> MSGQFTGTGTGGDVFKVDLNEQFDRADMVWIGTASVLVWIMIPGVGLLYSGISRKKHALSLMWAALMAACVAAFQWFWWGYSLVFAHNGSVFLGTLQNFCLKDVLGAPSIVKTVPDILFCLYQGMFAAVTAILMAGAGCERARLGPMMVFLFIWLTVVYCPIAYWTWGGNGWLVSLGALDFAGGGPVHENSGFAALAYSLWLGKRHDPVAKGKVPKYKPHSVSSIVMGTIFLWFGWYGFNGGSTGNSSMRSWYACVNTNLAAATGGLTWMLVDWFRTGGKWSTVGLCMGAIAGLVGITPAAGYVPVYTSVIFGIVPAIICNFAVDLKDLLQIDDGMDVWALHGVGGFVGNFMTGLFAADYVAMIDGTEIDGGWMNHHWKQLGYQLAGSCAVAAWSFTVTSIILLAMDRIPFLRIRLHEDEEMLGTDLAQIGEYAYYADDDPETNPYVLEPIRSTTISQPLPHIDGVADGSSNNDSGEAKNHHHHHH

structures of the Mep2 transceptors from S. cerevisiae and C. albicans. function as ammonium receptors/sensors in fungal development. a central channel for the transport of ammonium. non-phosphorylated, with channels that are closed on the cytoplasmic side.

different crystal forms to high resolution (up to 1.5 Å). Mep2 channel closure is likely due to movements of the CTR and ICL1 and ICL3. twin-His motif via hydrogen bonding with a highly conserved tyrosine hydroxyl group. the region beyond Ser457 is disordered. should facilitate the phosphorylation by Npr1. that the crystallization process favours closed states of the Mep2 channels. do show that Mep2 proteins can assume different conformations.> NPSYQQSPRHFVPTGMHSLALGTNLVEPLHALRLDAAGTTQHPVGCAPDEDMTVSSIASRYGLIRRVQWKKDHAKGSLLLQLDADPFVEQRIEGTNPISLYWFAPVGVVSSMFMQWRGSLEYRFDIIASQFHTGRLIVGYVPGLTASLQLQMDYMKLKSSSYVVFDLQESNSFTFEVPYVSYRPWWVRKYGGNYLPSSTDAPSTLFMYVQVPLIPMEAVSDTIDINVYVRGGSSFEVCVPVQPSLGLNWNTDFILRNDEEYRAKTGYAPYYAGVWHSFNNSNSLVFRWGSASDQIAQWPTISVPRGELAFLRIKDGKQAAVGTQ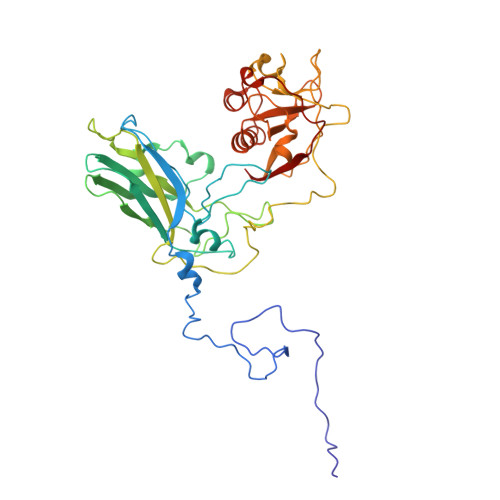PWRTMVVWPSGHGYNIGIPTYNAERARQLAQHLYGGGSLTDEKAKQLFVPANQQGPGKVSNGNPVWEVMRAPL> PAQDNSRFVIRDRNWHPKALTPDYKTSIARSPRQALVSIPQSISETTGPNFSHLGFGAHD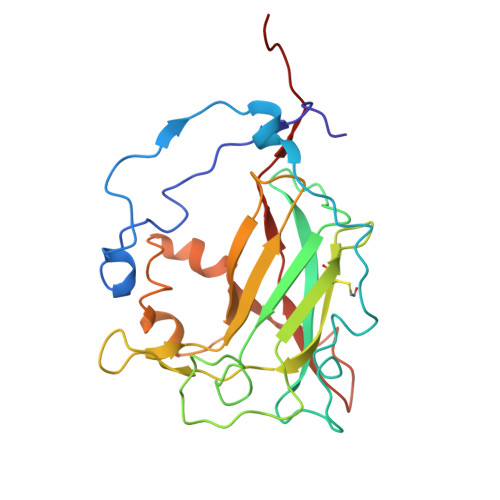HDLLLNFNNGGLPIGERIIVAGRVVDQYGKPVPNTLVEMWQANAGGRHRHKNDRYLAPLDPNFGGVGRCLTDSDGYYSFRTIKPGPYPWRNGPNDWRPAHIHFGISGPSIATKLITQLYFEGDPLIPMCPIVKSIANPEAVQQLIAKLDMNNANPMDCLAYRFDIVLRGQRKTHFENC>MSGMSPYKKAIEITKRLLELLLSNPELAKKNLGGIATLISLLALISALDGTLDEKDIEPYIKKLEESLGS[2x]

Here we use deep network hallucination to generate a wide range of symmetric protein homo-oligomers given only a specification of the number of protomers and the protomer length. Starting from only a choice of chain length L and oligomer valency N (2 for a dimer, 3 for a trimer, etc.), the method carries out a Monte Carlo search in sequence space starting from a random sequence. The loss function guiding the search is computed by inputting N copies of the sequence into the AlphaFold2 (AF2) network, and combining structure prediction confidence metrics (pLDDT; per-residue structural accuracy, and pTM; an estimate of the TM-score) with a measure of cyclic symmetry (the standard deviation of the distances between the center of mass of adjacent protomers within the predicted structure). To eliminate such over-fitting, we generated new sequences for the HAL backbones using the recently developed ProteinMPNN sequence design neural network (accompanying manuscript: Dauparas et al.).

To evaluate design accuracy we attempted crystallization of 19 designs and succeeded in solving crystal structures for seven (three C2s, two C3s and two C4s). All crystal structures had the correct oligomerization state and closely matched the design models (median Cα RMSD of 0.6 Å across all designs, with resolutions ranging from 1.8 to 3.4 Å). The side chain conformations in the crystal structures also closely match those of the design models. HALC4_136 is composed of 3-helix protomers with eight outer helices encasing four almost fully hydrophobic inner helices, where two of the helices are rigidly linked through a 90° helical kink. The closest match in the PDB has a TM-score of 0.71, but the matched structure has C5 symmetry rather than the C4 symmetry of the design and crystal structure.>GSSGSSGMVTDYSPEWSYPEGGVKVLITGPWQEASNNYSCLFDQISVPASLIQPGVLRCYCPAHDT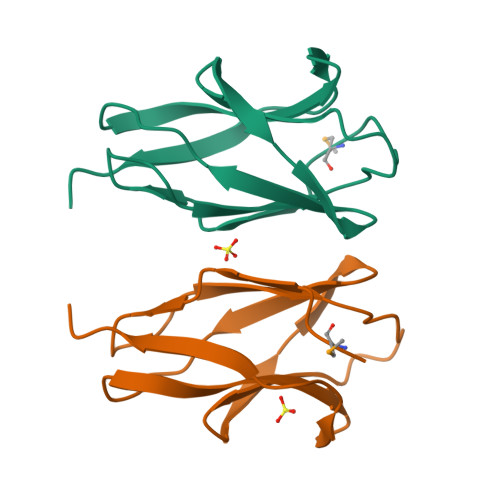GLVTLQVAFNNQIISNSVVFEYKSGPSSG[5x]>[2x]MYSRADRLLRQFSLKLNTDSIVFDENRLCSFIIDNRYRILLTSTNSEYIMIYGFCGKPPDNNNLAFEFLNANLWFAENNGPHLCYDNNSQSLLLALNFSL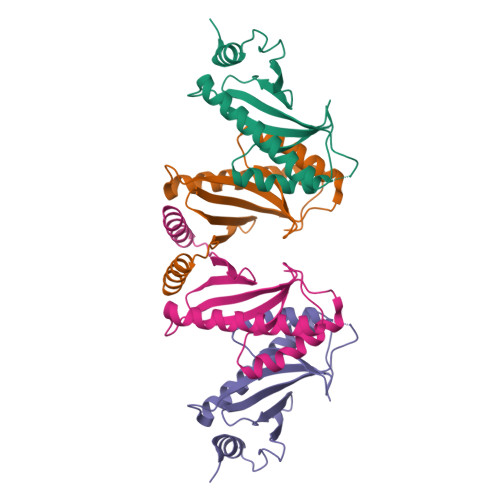NESSVEKLECEIEVVIRSMENLYHILQDKGITLDTDYTHHHHHH>[2x]SNMLDYKKYEGQTRGELIWSRLNPLRHTAKMSMARAQLITDGYKEYEGYSLYRKRGLSVRKIMREIPIFIDDDQLLVGDFSATQMSPEWYPDLAASWVEDYIDKYGWKGSGTFYEFTGPEQAEQARAIAQYWHNIGGKEMWIKYMGPEQEEFEAKIGEAGGYLTNTVSEMYAEKAWNVPDCARMITTGARGFIEEIDNKLANLTVLTDEDYRAHEFYLALRYELEGVIDYAHRYAALAREKAAVERDPQRKVELEEIARVCDRVPEYPAETFQEALQSFFFAVLMVYWDTRTYGMGMGRMDQFLYPTFKKDIERGYIDEKYAQDLLECFRCKIMEKRQFWPDVMVPSVSAESHFHNVVLGGVDPKTGKDATNRLSYLFLDAATKVRTPHPTLSVRWHANIDEKFMDRALEVVAMGMGFPAFFGDDTTIQYLLERGYTLEEARNYAIGGCVLHQVPGKQSSVWPIVQNYGKMLEMTLNNGFNWYSQEQIGPKTG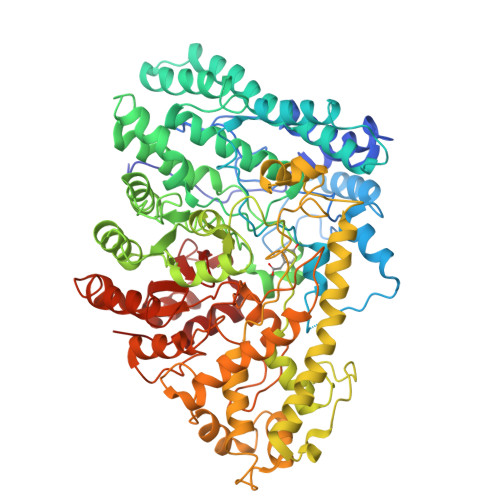NFLEMKTYDEFIEAYRKQCEYWAQIAANSNRQCRIEHLESFPDIAMSCFVDDCIDRGKVCSLGGAAHNDNTQYIVPVGVQDLGNNLYVLKNQIFVDNPICSKETLLDAIHKNWEGYEDLQAKMIAMPKFGNDIPEVDELVNWGYKFIEDIWFKIPSAYGSHFEVAPHSIGFHAGTGAKCSALPDGRVAWTAMSDGAVSPRQGTDTNGPAAVMCSAGCVDQVDLFGVLFNMRFTPQSLADKSGRDKLKALIETYFHDMGGKHVQFNVMSKKQMIEAKEHPLEHQDLIVRVAGYSAYWADLSTTIQDELIARSELTI> DYKDDDDKMVFEQHEEEAVAPGAVHGHRLSTVVPSSVTGEVDYALADADLAFKLHYLRGVYYYRSGDGLATKVLKDPMFPWLDDHFPVAGRVRRAEAEGDGAPRRPYIKCNDCGVRIVEARCDRDMAEWIRDAAPGRIRQLCYDKVLGPELFFSPLLYVQITNFKCGGLALGFSWAHLIGDIPSAATCFNKWAQILSGKKPEATVLTPPNQ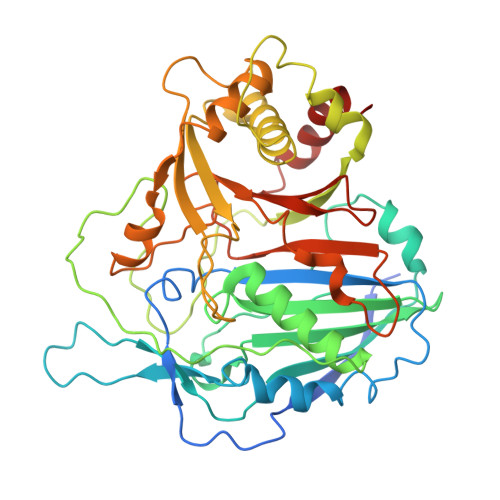PLQGQSPAAPRSVKQVGPMEDLWLVPAGRDMACYSFHVSDAVLKKLHQQQNGRQDAAAGTFELVSALVWQAVAKIRGDVDTVTVVRADAAARSGKSLANEMKVGYVESAGSSPAKTDVAELAALLAKNVVDETAAVAAFQGDVLVYGGANLTLVDMEQVDLYGLEIKGQRPVYVEYGMDGVGDEGAVLVQPDADGRGRLVTVVLPGDEIDSLRAALGSALHVA>GTENLYFQGMSDVIEGRLKELGFTLPVAAAPAANYVPFTISGNLLYVSGQLPMESGKIAVTGLVGRDVDVASAQRAAELCAVNILAQVKAALNGDLSKIRRVIKLNGFVASVPEFVEQHLVINGASNLIATVLGEPGRHARAAVGMASLPFNASVEIDAIV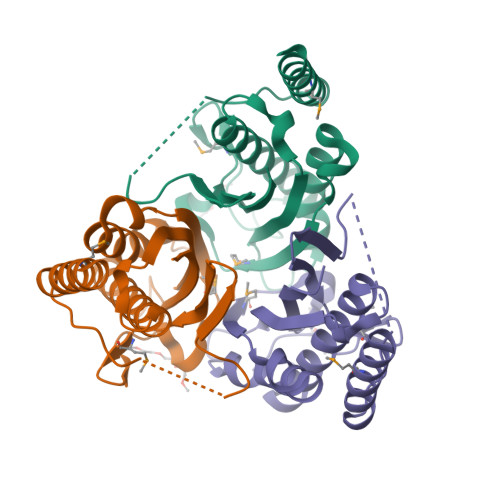EIDV[12x]> GPHMASAEEKLEKKLELDPNCKEPLQVLPPTVVDQIRLWQLELDRVITYEGSLYSDFETSQE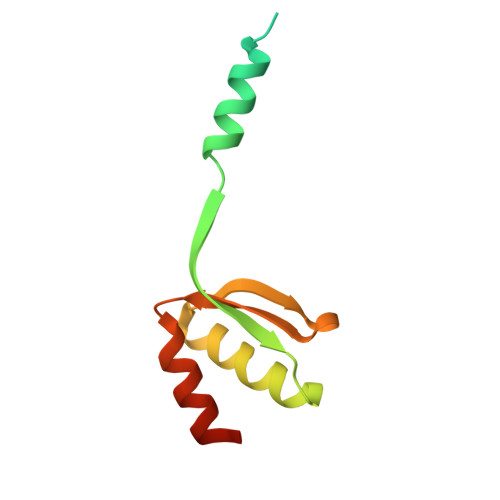YNLLSKYAQDIGVLLWKDDKKKKFFISKEGNSQVLDFAKRKLKKKQ> MKGFFAGVVAAATLAVASAGDYCGQWDWAKSTNYIVYNNLWNKNAAASGSQCTGVDKISGSTIAWHTSYTWTGGAATEVKSYSNAALVFSKKQIKNIKSIPTKMKYSYSHSSGTFVADVSYDLFTSSTASGSNEYEIMIWLAAYGGAGPISSTGKAIATVTIGSNSFKLYKGPNGSTTVFSFVATKTITNFSADLQKFLSYLTKNQGLPSSQYLITLEAGTEPFVGTNAKMTVSSFSAAVN;> MGKREYPSSAHFLVTLSLLLLQAAFGLTLCIEKERDALLEFKRGLSDNFGQLSTWGDEEDKKECCKWKGIECNKTTGHVIVLDLHNAFTCSASACFAPRLTGKLSPSLLELEYLNFLDLSVNEFERSEIPRFICSFKRLEYLNLSSSFFSGLIPTQFKNLTSLRILDLGYNNLIVKDLTWLSHLSSLELLSLGGSDFQVKNWFQEITKLPLLKELDLSLCGLSKLVPSPAEIANSSLISLSVLHLCCNEFSSSAKYSWLFNFSTSLTSIDLSNNQLDGQIDDRFGNLMYLEHLNLANELNLKGGIPSSFGNLTRLRYLDMSNTRTYQWLPELFVRLSGSRKTLEVLGLNDNSMFGSLVDVTRFSALKRLYLQKNVLNGFFMERFGQVSSLEYLDLSDNQM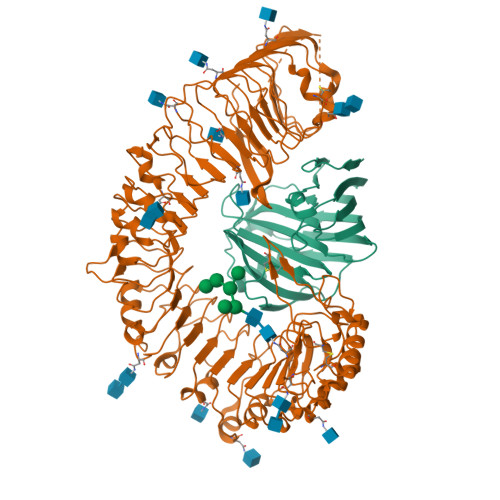RGPLPDLALFPSLRELHLGSNHFNGRIPQGIGKLSQLKILDVSSNRLEGLPESMGQLSNLESFDASYNVLKGTITESHLSNLSSLVDLDLSFNSLALKTSIDWLPPFQLQVINLPSCNLGPSFPKWLQSQNNYTVLDISLANISDALPSWFSGLPPDIKILNLSNNQISGRVSDLIENAYDYMVIDLSSNNFSGPLPLVPTNVQIFYLHKNQFFGSISSICKSTTGATSLDLSHNQFSGELPDCWMNATNLAVLNLAYNNFSGKLPQSLGSLTNLEALYMRQNSFSGMLPSLSQCQSLQILDLGGNKLTGRIPAWIGTDLLNLRILSLRFNKFYGSISPIICQLQFLQILDLSANGLAGKIPQCFNNFTLLHQENGLGEPMEFLVQGFYGKYPRHYSYLGNLLVQWKNQEAEYKNPLTYLKTIDLSSNKLVGGIPKEMAEMRGLKSLNLSRNDLNGSIIKGIGQMKMLESLDLSRNQLSGMIPKDLANLTFIGVLDLSNNHLSGRIPSSTQLQTFERSSYSGNAQLCGPPLQEC>[2x]MYMKHIENGTRIEGEYIKNKVIQYNMSILTDEVKQPMEEVSLVV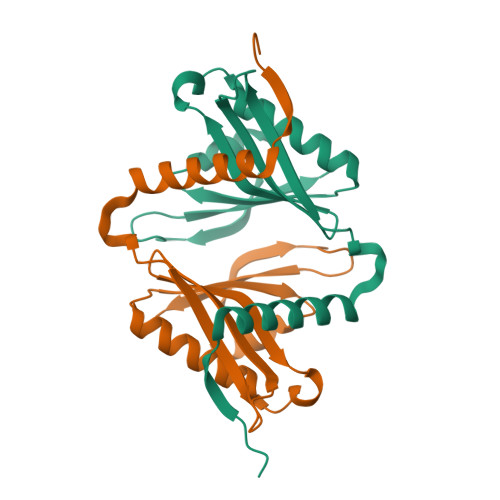KNEEGKIFGGVTGTMYFYHLHIDFLWVDESVRHDGYGSQLLHEIEGIAKEKGCRLILLDSFSFQAPEFYKKHGYREYGVVEDHPKGHSQHFFEKRL> MRGSHHHHHHGIHMNSLIKENMRMMVVMEGSVNGYQFKCTGEGDGNPYMGTQTMRIKVVEGGPLPFAFDILATSFMYGSKTFIKHTKGIPDFFKQSFPEGFTWERVTRYEDGGVFTVMQDTSLEDGCLVYHAKVTGTNFPSNGAVMQKKTKGWEPNTEMLYPADGGLRGY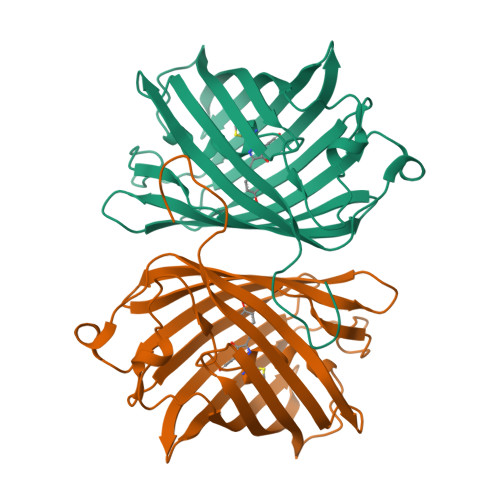SQMALNVDGGGYLSCSFETTYRSKKTVENFKMPGFHFVDHRLERLEESDKEMFVVQHEHAVAKFCDLPSKLGRL> DLEELEQFAKTFKQRRIKLGFTQGDVGLAMGKLYGNDFSQTTISRFEALNLSFK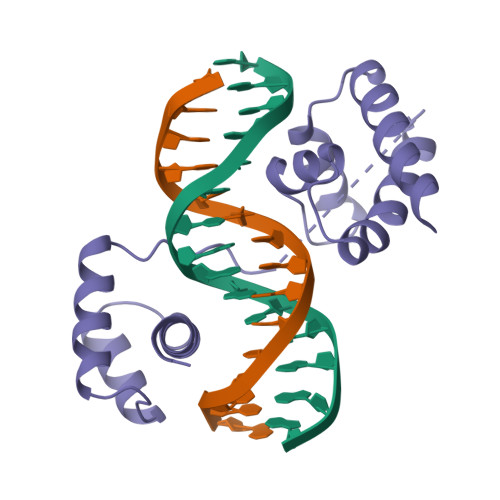NMCKLKPLLEKWLNDAENLSSDSSLSSPSALNSPGIEGLSRRRKKRTSIETNIRVALEKSFLENQKPTSEEITMIADQLNMEKEVIRVWFCNRRQKEKRINP>[3x]MVCKVCGQKAQVEMRSRGLALCREHYLDWFVKETERAIRRHRMLLPGERVLVAVSGGKDSLALWDVLSRLGYQAVGLHIELGIGEYSKRSLEVTQAFARERGLELLVVDLKEAYGFGVPELARLSGRVACSACGLSKRYIINQVAVEEGFRVVATGHNLDDEAAVLFGNLLNPQEETLSRQGPVLPEKPGLAARVKPFYRFSEREVLSYTLLRGIRYLHEECPNAKGAKSLLYKEALNLVERSMPGAKLRFLDGFLEKIRPRLDVGEEVALRECERCGYPTTGAVCAFCRMWDAVYRRAKKRKLLPEEVSFRPRVKPLRAG;>MGSSHHHHHHRVVLRLPERKEVEVKGNRPLREVLEELGLNPETVVAVRGEELLTLEDEVREEDTLEVLSAISGG[3x]

TtuA transfers sulfur from sulfur donor TtuB to substrate tRNA by consuming ATP. The enzymatic activity of TtuA is dependent on a [4Fe-4S] cluster. TtuB is a ubiquitin-like protein with a molecular mass of ~7 kDa. Only three cysteine residues chelate the cluster, leaving one Fe atom (hereafter referred to as the unique Fe site) remaining free from coordination by TtuA.

The crystal structure of holo-TtuA in complex with TtuB-COOH and adenosine triphosphate (ATP) was successfully determined at 2.2 Å resolution. The manner of interactions between TtuA and Fe-S (i.e., TtuA coordinately bound to Fe-S via three cysteine residues) was identical to that for holo-TtuA reported previously. However, a new interaction directly coordinated between the unique Fe site of the [4Fe-4S] cluster and the C-terminus of TtuB was observed. One of the three TtuA–TtuB heterodimers in one asymmetric unit showed the electron density of the Fe-S cluster connected to the C-terminus of TtuB, indicating coordinate binding of TtuB to the Fe-S cluster. Distinct from other Fe atoms belonging to the Fe-S cluster, which are tetrahedrally coordinated, the unique Fe site is octahedrally coordinated to the C-terminal of TtuB. Two oxygen atoms from TtuB and two sulfur atoms from the Fe-S cluster form the equatorial plane of the octahedron. The distance between each of the two oxygen atoms and the unique Fe site was 2.4 and 2.5 Å, respectively. Along the axis of the octahedron, a water molecule was detected ~3.7 Å from the unique Fe site. On this axis, Lys137 of TtuA lies across the water molecule and forms a hydrogen bond with it. Based on the similarity of the chemical structure of the carboxyl (-COOH) and thiocarboxyl (-COSH) groups, the structure of TtuA–TtuB(COOH) is considered to mimic the state of TtuB-COSH coordinated by the unique Fe site after forming the TtuA–TtuB complex.>[2x]GTLTGERPPVFWLQGQGCTGCSVTLLNSVHPSIADVLLKVISLEFHPTVMAWEGEHAIEHMRKVAEKFKGKFFLVIEGSVPVEADGKYCIIGEANHHEISMVDALKEFGPNAAAVLAVGTCAAYGGIPAAEGSETGATAVSKFLGDNGIKTPVVNIPGCPPHPDWIVGTVVLALDAIKKNGLEGGLAEVVKVLDSDGRPTPFFGRNIHENCPYLDKYDEGVMSATFTDKVGCRYDLGCKGPMTMADCFERKWNGGVNWCVQNAVCIGCVEPDFPDGKSPFYQA;>[2x]GATGRTTIAIDPVTRIEGHLKAEVVVENGKVVDARLSGGMYRGFETILRGRDPRDASQIVQRICGVCPTAHSTASVLALDEAFGAKVPNNGRITRNLIFGANYLQSHILHFYHLSAQDFVQGPDTAPFVPRFPKSDLRLSKELNKAGVDQYIEALEVRRICHEMVALFGGRMPHVQGQVVGGATEIPTKEKLVEYAAR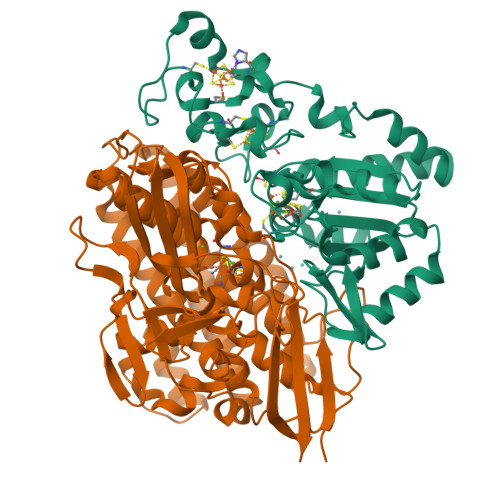FKKVRDFVEQKYVPVVYTIGSKYKDMFKVGQGFKAALCVGAFPLDNSGKKHLFMPGVYAKGKDMPFDPSKIKEYVKYSWFAEETTGLNYKEGKTIPAPDKAGAYSFVKAPRYDGLSLEVGPLARMWVNNPELSPVGKKLLKDLFGISAKKFRDLGEEAAFSLMGRHVARAEETYYMLGAIEGWLKEIKAGEDTVVMPAVPASAEGTGFTEAPRGSLLHYVKVKDSKIDNYQIVSASLWNCNPRDDMGQRGAVEEALIGIPVDDIQNPVNVARLIRAFDPULACAVH1,3,5-triazine-2,4,6-triamine | 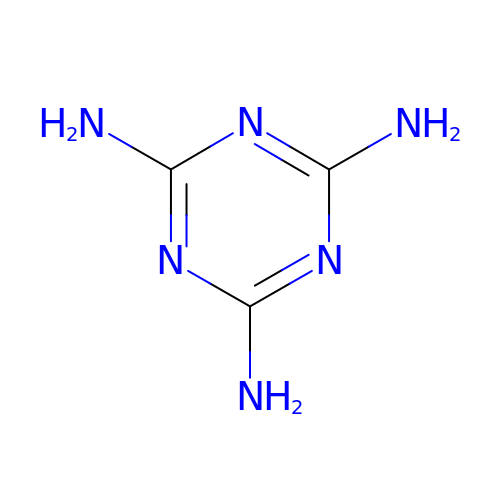C3 H6 N6 | JDSHMPZPIAZGSV-UHFFFAOYSA-N>[4x]GHMIARGKFRSLTLINWNGFFARTFDFDELVTTLSGGNGAGKSTTMAGFVTALIPDLTLLNFRNTTEAGSTSSSRDKGLYGKLKAGVCYAVLETVNSRAQRIITGVRLQQIAGRDKKVDIRPFSLQNVPMTDSVISLFTEQVANKARVLSLNDLKEKFEETAVTFKPYHSITDYHSFMFDLGILPKRLRSSSDRNKFYKLIEASLYGGISSVITKSLRDYLLPENSGVRQAFQDMEAALRENSGGSGGSISAESVANILR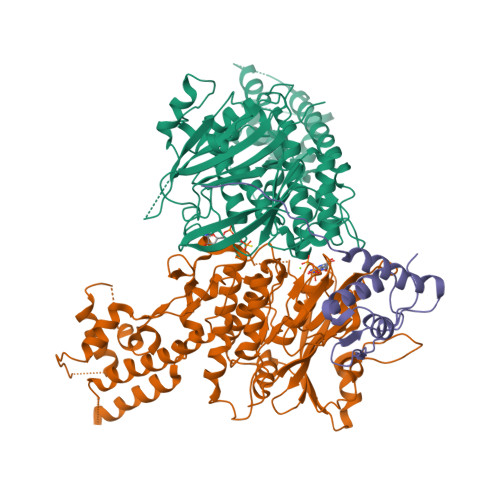KTIQREQNRILQLNQGLQNIAFGQVKGVRLVVNIRDTHSILLNALSDQHEQHKDLFESQKLSFSEALAMLYKRINPHIELGQRMPQTIGEELLDYRNYLDLEVETLRGAYGWMRAESSALSTGEAIGTGMSILLMVVQSWEEESRRMRAKDILPCRLLFLDQAARLDAMSINTLFELCERLDMQLLIAAPENISPERGTTYKLVRKILANQEYVHVVGLKGFG;>[2x]MDKNRVFGQRLRQSIQNYFSSPWLLYTAKAEALLDLRDDEAMLNEMEAVGELPMALEYESLTDVQTQIVTAIQAELAHFRNTAQPINLGAVLQEQLARYPQSRHFDVARIIVDQAVKLGMASQDHQAVYPVWQPIDDFSAAVQAHLIDQYDK;>[2x]MTEYIQDAIPAKLAIAIANPIFPQLDSQLRAGRHISIEMLDEHAFLMDFQTELESFYRRYHVDLIRAPEGFFYLRPKASTLIARSAMSEMEMLVGKVLCYLYLSPERLAQQGIFSQDDVYEELLNLADENKLLKAVNPRSTGSDLDRAKLAEKVGGALRRLARIGIITRVGEQNSKKFIISEAVFRFGADVRAGDDPREVQLRLIRDGEATTPTLLTTAAIEFAEDGARDELEESEAE>MSLSVAIIGPGAVGTTIAYELQQSLPHTTLIGRHAKTITYYTVPHAPAQDIVVKGYEDVTNTFDVIIIAVKTHQLDAVIPHLTYLAHEDTLIILAQNGYGQLEHIPFKNVCQAVVYISGQKKGDVVTHFRDYQLRIQDNALTRQFRDLVQDSQIDIVLEANIQQAIWYKLLVNLGINSITALGRQTVAIMHNPEIRILCRQLLLDGCRVAQAEGLNFSEQTVDTIMTIYQGYPDEMGTSMYYDIVHQQPL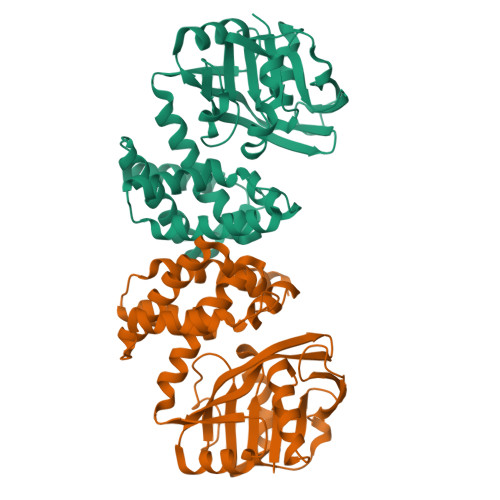EVEAIQGFIYRRAREHNLDTPYLDTIYSFLRAYQQNEGHHHHHH[8x]> GFTDYKVADITLAAWGRRELIIAESEMPALMGLRRKYAGQQPLKGAKILGCIHMTIQTGVLIETLVALGAEVRWSSCNIFSTQDQAAAAIAAAGIPVFAWKGETEEEYEWCIEQTILKDGQPWD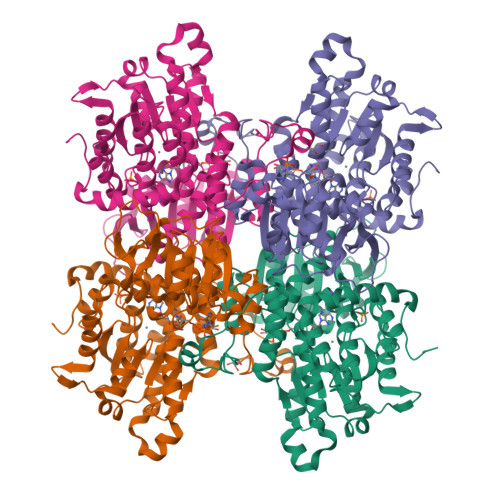ANMVLDDGGDLTEILHKKYPQMLERIHGITEETTTGVHRLLDMLKNGTLKVPAINVNDSVTKSKNDNKYGCRHSLNDAIKRGTDHLLSGKQALVIGYGDVGKGSSQSLRQEGMIVKVAEVDPICAMQACMDGFEVVSPYKNGINDGTEASIDAALLGKIDLIVTTTGNVNVCDANMLKALKKRAVVCNIGHFDNEIDTAFMRKNWAWEEVKPQVHKIHRTGKDGFDAHNDDYLILLAEGRLVNLGNATGHPSRIMDGSFANQVLAQIHLFEQKYADLPAAEKAKRLSVEVLPKKLDEEVALEMVKGFGGVVTQLTPKQAEYIGVSVEGPFKPDTYRY;>[3x]FTDYKVADITLAAWGRRELIIAESEMPALMGLRRKYAGQQPLKGAKILGCIHMTIQTGVLIETLVALGAEVRWSSCNIFSTQDQAAAAIAAAGIPVFAWKGETEEEYEWCIEQTILKDGQPWDANMVLDDGGDLTEILHKKYPQMLERIHGITEETTTGVHRLLDMLKNGTLKVPAINVNDSVTKSKNDNKYGCRHSLNDAIKRGTDHLLSGKQALVIGYGDVGKGSSQSLRQEGMIVKVAEVDPICAMQACMDGFEVVSPYKNGINDGTEASIDAALLGKIDLIVTTTGNVNVCDANMLKALKKRAVVCNIGHFDNEIDTAFMRKNWAWEEVKPQVHKIHRTGKDGFDAHNDDYLILLAEGRLVNLGNATGHPSRIMDGSFANQVLAQIHLFEQKYADLPAAEKAKRLSVEVLPKKLDEEVALEMVKGFGGVVTQLTPKQAEYIGVSVEGPFKPDTYRY> 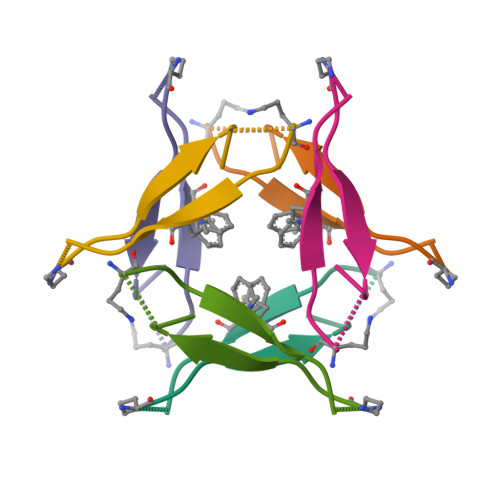VAKLVFFAKAAIIGLM> SMPK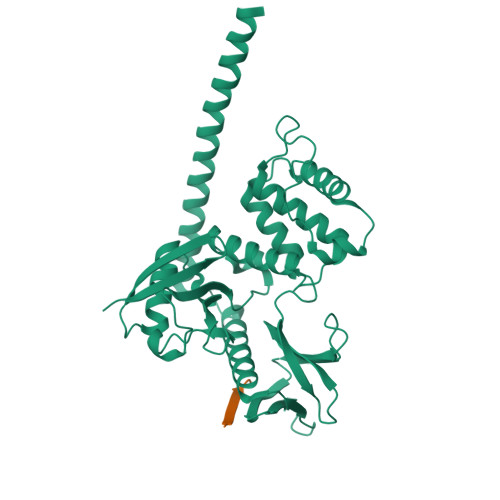TISVRVTTMDAELEFAIQPNTTGKQLFDQVVKTIGLREVWFFGLQYQDTKGFSTWLKLNKKVTAQDVRKESPLLFKFRAKFYPEDVSEELIQDITQRLFFLQVKEGILNDDIYCPPETAVLLASYAVQSKYGDFNKEVHKSGYLAGDKLLPQRVLEQHKLNKDQWEERIQVWHEEHRGMLREDAVLEYLKIAQDLEMYGVNYFSIKNKKGSELWLGVDALGLNIYEQNDRLTPKIGFPWSEIRNISFNDKKFVIKPIDKKAPDFVFYAPRLRINKRILALCMGNHELYMRRRKPDTIEVQQMKAQAREEKHQKQMERAMLENEKKKREMAEKEKEKIEREKEE;> QKKKLVIN>[2x]MSNLVLY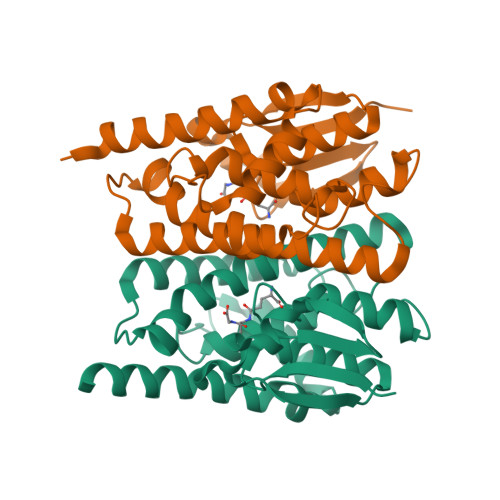TLHLSPPCRAVELTAKALGLELEQKTINLLTGDHLKPEFVKLNPQHTIPVLDDNGTIITESHAIMIYLVTKYGKDDSLYPKDPVKQARVNSALHFESGVLFARMRFIFERILFFGKSDIPEDRVEYVQKSYELLEDTLVDDFVAGPTMTIADFSCISTISSIMGVVPLEQSKHPRIYAWIDRLKQLPYYEEANGGGGTDLGKFVLAKKEENAKA>[2x]MSLSYLTEEKLTIVGAAGMIGSNMAQTAAMMRLTPNLCLYDPFAVGLEGVAEEIRHCGFEGLNLTFTSDIKEALTDAKYIVSSGGAPRKEGMTREDLLKGNAEIAAQLGKDIKSYCPDCKHVIIIFNPADITGLVTLIYSGLKPSQVTTLAGLDSTRLQSELAKHFGIKQSLVTNTRTYGGHGEQMAVFASTAKVNGTPLTDLIGTDKLTNEQWAELKQRVVKGGANIIKL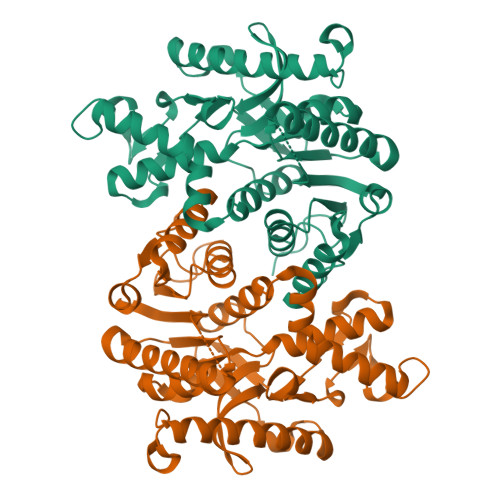RGRSSFQSPSYVSIEMIRAAMGGEAFRWPAGCYVNVPGFEHIMMAMETTITKDGVKHSDINQLGNEAERAALKESYSHLAKLRDEVIAMGIIPAIADWKTVNPNEGHHHHHH> MAQILPIRFQEHLQLQNLGINPANIGFSTLTMESDKFICIREKVGEQAQVVIIDMNDPSNPIRRPISADSAIMNPASKVIALKAGKTLQIFNIEMKSKMKAHTMTDDVTFWKWISLNTVALVTDNAVYHWSMEGESQPVKMFDRHSSLAGCQIINYRTDAKQKWLLLTGISAQQNRVVGAMQLYSVDRKVSQPIEGHAASFAQFKMEGNAEESTLFCFAVRGQAGGKLHIIEVGTPPTGNQPFPKKAVDVFFPPEAQNDFPVAMQISEKHDVVFLITKYGYIHLYDLETGTCIYMNRISGETIFVTAPHEATAGIIGVNRKGQVLSVCVEEENIIPYITNVLQNPDLALRMAVRNNLAGAEELFARKFNALFAQGNYSEAAKVAANAPKGILRTPDTIRRFQSVPAQPGQTSPLLQYFGILLDQGQLNKYESLELCRP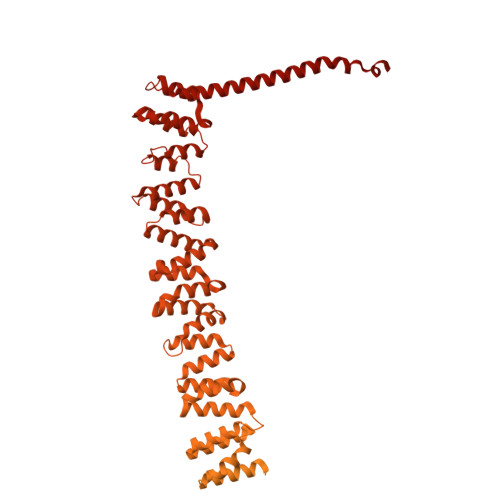VLQQGRKQLLEKWLKEDKLECSEELGDLVKSVDPTLALSVYLRANVPNKVIQCFAETGQVQKIVLYAKKVGYTPDWIFLLRNVMRISPDQGQQFAQMLVQDEEPLADITQIVDVFMEYNLIQQCTAFLLDALKNNRPSEGPLQTRLLEMNLMHAPQVADAILGNQMFTHYDRAHIAQLCEKAGLLQRALEHFTDLYDIKRAVVHTHLLNPEWLVNYFGSLSVEDSLECLRAMLSANIRQNLQICVQVASKYHEQLSTQSLIELFESFKSFEGLFYFLGSIVNFSQDPDVHFKYIQAACKTGQIKEVERICRESNCYDPERVKNFLKEAKLTDQLPLIIVCDRFDFVHDLVLYLYRNNLQKYIEIYVQKVNPSRLPVVIGGLLDVDCSEDVIKNLILVVRGQFSTDELVAEVEKRNRLKLLLPWLEARIHEGCEEPATHNALAKIYIDSNNNPERFLRENPYYDSRVVGKYCEKRDPHLACVAYERGQCDLELINVCNENSLFKSLSRYLVRRKDPELWGSVLLESNPYRRPLIDQVVQTALSETQDPEEVSVTVKAFMTADLPNELIELLEKIVLDNSVFSEHRNLQNLLILTAIKADRTRVMEYINRLDNYDAPDIANIAISNELFEEAFAIFRKFDVNTSAVQVLIEHIGNLDRAYEFAERCNEPAVWSQLAKAQLQKGMVKEAIDSYIKADDPSSYMEVVQAANTSGNWEELVKYLQMARKKARESYVETELIFALAKTNRLAELEEFINGPNNAHIQQVGDRCYDEKMYDAAKLLYNNVSNFGRLASTLVHLGEYQAAVDGARKANSTRTWKEVCFACVDGKEFRLAQMCGLHIVVHADELEELINYYQDRGYFEELITMLEAALGLERAHMGMFTELAILYSKFKPQKMREHLELFWSRVNIPKVLRAAEQAHLWAELVFLYDKYEEYDNAIITMMNHPTDAWKEGQFKDIITKVANVELYYRAIQFYLEFKPLLLNDLLMVLSPRLDHTRAVNYFSKVKQLPLVKPYLRSVQNHNNKSVNESLNNLFITEEDYQALRTSIDAYDNFDNISLAQRLEKHELIEFRRIAAYLFKGNNRWKQSVELCKKDSLYKDAMQYASESKDTELAEELLQWFLQEEKRECFGACLFTCYDLLRPDVVLETAWRHNIMDFAMPYFIQVMKEYLTKVDKLDASESLRKEEEQATETQPIVYGQPQLMLTAGPSVAVPPQAPFGYGYTAPAYGQPQPGFGYSM> MIIIRYLVRETLKSQLAILFILLLIFFCQKLVRILGAAVDGDIPANLVLSLLGLGVPEMAQLILPLSLFLGL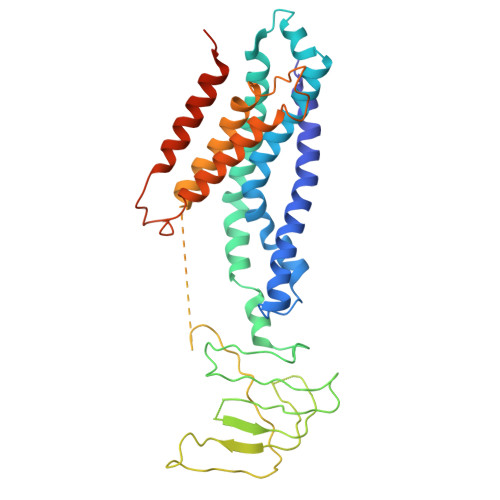LMTLGKLYTESEITVMHACGLSKAVLVKAAMILAVFTAIVAAVNVMWAGPWSSRHQDEVLAEAKANPGMAALAQGQFQQATNGSSVLFIESVDGSDFKDVFLAQIRPKGNARPSVVVADSGHLTQLRDGSQVVTLNQGTRFEGTALLRDFRITDFQDYQAIIGHQAVALDPNDTDQMDMRTLWNTDTDRARAELNWRITLVFTVFMMALMVVPLSVVNPRQGRVLSMLPAMLLYLLFFLIQTSLKSNGGKGKLDPTLWMWTVNLIYLALAIVLNLWDTVPVRRLRASFSRKGAV2-RIBOFURANOSYL-3-IODO-2,3-DIHYDRO-1H-PYRAZOLO[3,4-D]PYRIMIDIN-4-YLAMINE 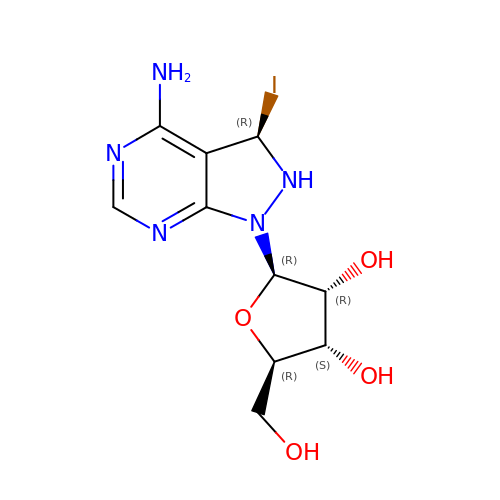| C10 H14 I N5 O4 | IPMOTTQXPAXTMS-CKVFBBIQSA-N> MRSPAAFVARSGLFKASLGQSNWAQKAEQMMASVTRTFAADAKALDELRKPKFSSKYLIQHVSQKLIPAVKEWEKSYQPPVIHLGRVLSVGDGIARVYGLKSVQAGELVCFDSGVKGMALNLQADHVGVVVFGNDSVIHQGDLVYRTGQIVNVPIGPGTLGRVTDG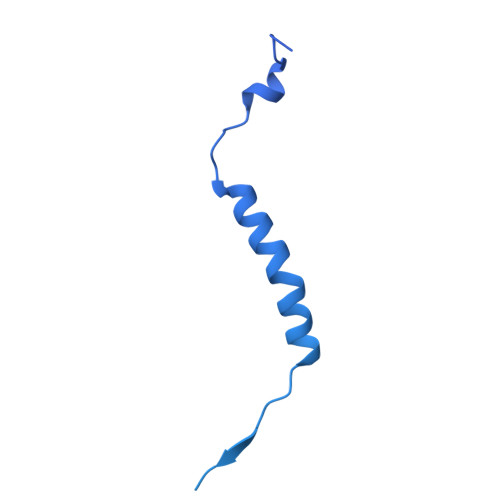LGQPIDGKGPLTNVRSSLVEVKAPGIIARQSVREPLFTGVKAVDALVPIGRGQRELIIGDRQTGKTAVAIDAIIHQKNCNEQVPKAQRVYCVYVAVGQKRSTVAQLVKLFTQTGAMRYTIMVSATASDAAPLQFLAPYSGCAMAEYFRDTGKHGLIIYDDLSKQSVAYRQMSLLLRRPPGREAFPGDVFYLHSRLLERAAKLSKELGGGSLTAFPVIETQAGDVSAYIATNVISITDGQIFLETELFYKGIRPALNVGLSVSRVGSAAQFPGMKQVAGTLKLELAQYREVAAFAQFGSDLDAATQYVLERGARLTEMLKQKQFAPIPIERQTVAVYAATKGFLDKVRVQDIVAAEEAVISQVNPAVFKILKANGKITPALDAHLKAELRKVKLPGA>MGSSHHHHHHSSMKQAILYVGHGSRVKKAQQEAAAFLEGCKAHISVPVQEISFLELQEPTIETGFEACVKQGATHIAVVPLLLLTAAHAKHDIPEEIVRVASRYPSVRISYGKPIGIDEEVVKAVYHRMKDIGVPYENARVVLIGRGSSDPDVKRDVTGIANLLQEMVPVKEVIPCFLTACGPNYKEVFSELEKDDGITTFIVPYLLFTGMLMNEIEREVQKLKAHNPNVYLSSYIGFHPHVKNAFLNRVRETAA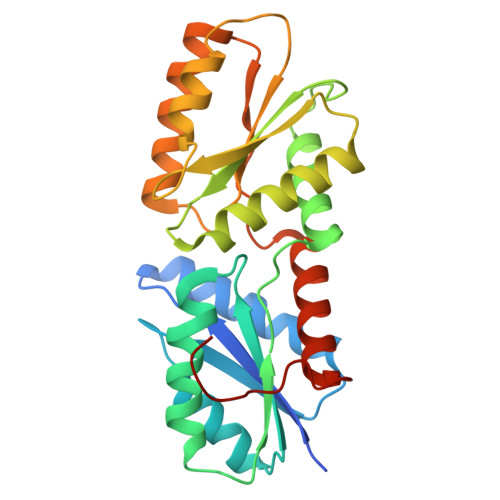NSEGQFDFDGGSYASAAH[2x]>[4x]VANPEHYIKHPLQNRWALWFFKNDKSKTWQANLRLISKFDTVEDFWALYNHIQLSSNL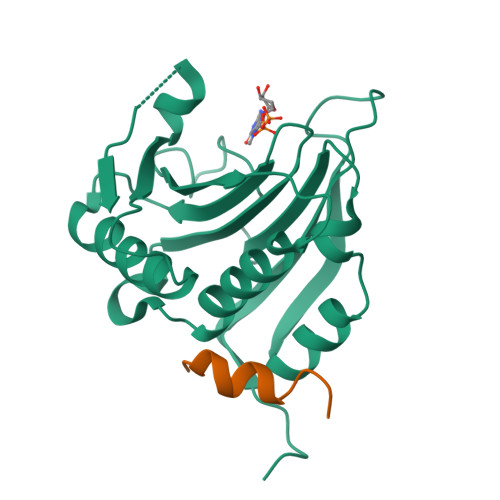MPGCDYSLFKDGIEPMWEDEKNKRGGRWLITLNKQQRRSDLDRFWLETLLCLIGESFDDYSDDVCGAVVNVRAKGDKIAIWTTECENRDAVTHIGRVYKERLGLPPKIVIGYQSHADTATKSGSTTKNRFVV;>[4x]KQYDREFLLDFQFMPA>MRFFLSPPHMGGNELKYIEEVFKSNYIAPLGEFVNRFEQSVKDYSKSENALALNSATAALHLALRVAGVKQDDIVLASSFTFIASVAPICYLKAKPVFIDCDETYNIDVDLLKLAIKECEKKPKALILTHLYGNAAKMDEIVEICKENDIVLIEDAAEALGSFYKNKALGTFGEFGVYSYNGNKIITTSGGGMLIGKNKEKIEKARFYSTQARENCLHYEHLDYGYNYRLSNVL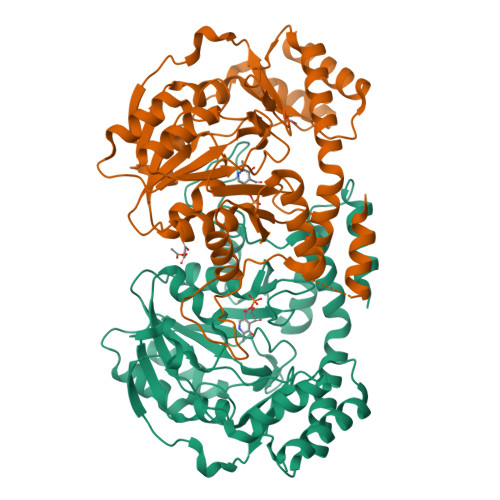GAIGVAQMEVLEQRVLKKREIYEWYKEFLGEYFSFLDELENSRSNRWLSTALINFDKNELNACQKDINISQKNITLHPKISKLIEDLKNKQIETRPLWKAMHTQEVFKGAKAYLNGNSELFFQKGICLPSGTAMSKDDVYEISKLILKSIKAGSHHHHHH[2x]> LK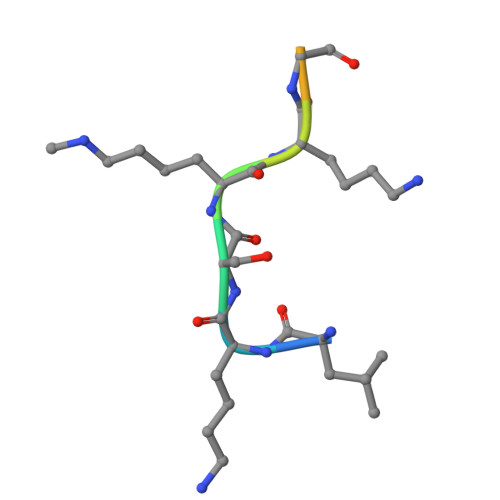SKKGQSTY> MSGELSNRFQGGKAFGILKARQERRLAEINREFLCDQKYSDEENLPEKLTAFKEKYMEFDLNNEGEIDLMSLKRMMEKLGVPKTHLEMKKMISEVTGGVSDTISYRDFVNMMLGKRSAVLKLVMMFEGKANESSPKPVG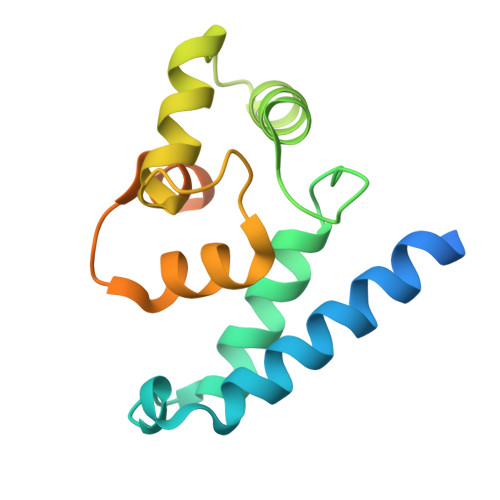PPPERDIASLP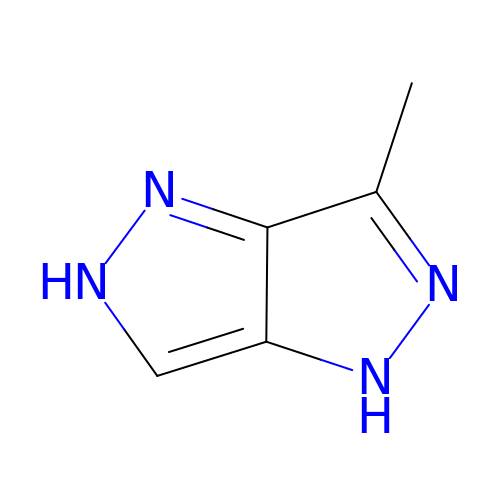3-methyl-1,5-dihydropyrazolo[4,3-c]pyrazole | C5 H6 N4 | KRAKREBEXWCQMF-UHFFFAOYSA-N> GTPRV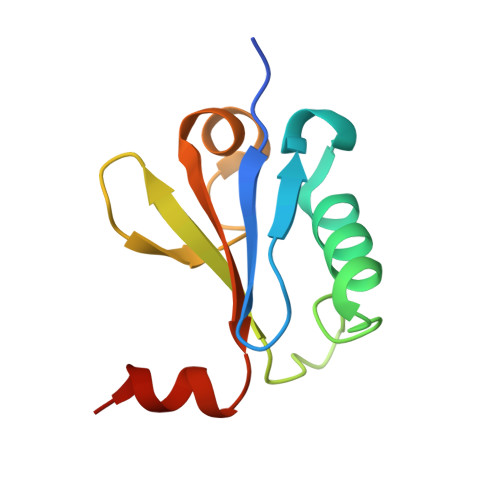RTYTDVQKTGSVGRSIDVTSFKDYEELKSAIESMFGLEGLLTHPQSSGWKLVYVDYESDVLLVGDDPWEEFVGSVRSIRILSPTEVQQMSEEG> MNRSVNIAKNLIQTYRAMSVQSRFAFSTREEEWLDKRTKSQEKVYFDQEDRKAMKRLLEKLNTT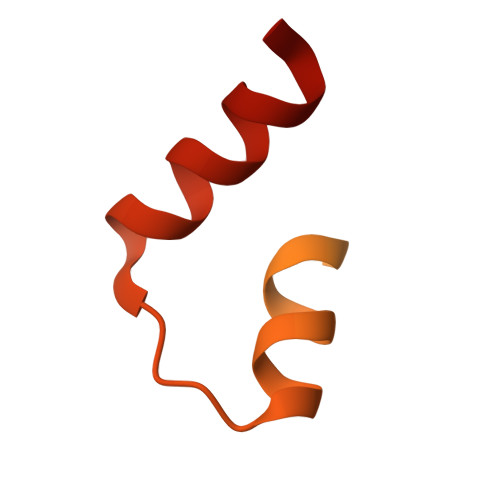SKFVEDSEYLAPQNLEVENILKRYHINYTQALIDELVDWKTGKN> VLAMSKIEIKLSDIPEGKNMAFKWRGKPL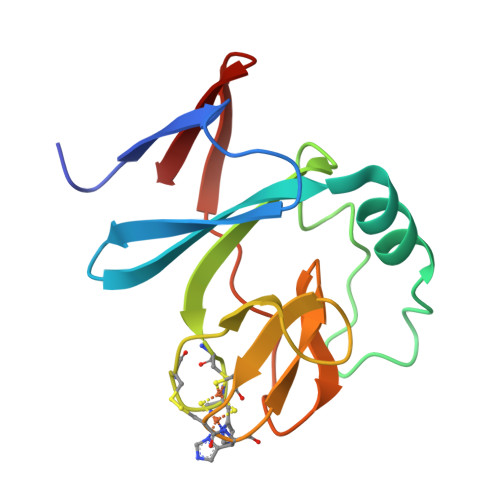FVRHRTKKEIDQEAAVEVSQLRDPQHDLERVKKPEWVILIGVCTHLGCVPIANAGDFGGYYCPCHGSHYDASGRIRKGPAPLNLEVPSYEFTSDDMVIVG>[2x]AKVFQWFGSNESGAEFGSQNLPGVEGKDYIWPDPNTIDTLISKGMNIFRVPFMMERLVPNSMTGSPDPNYLADLIATVNAITQKGAYAVVDPHNYGRYYNSIISSPSDFETFWKTVASQFASNPLVIFDTDNEYHDMDQTLVLNLNQAAIDGIRSAGATSQYIFVEGNSWTGAWTWTNVNDNMKSLTDPSDKIIYEMHQYLDSD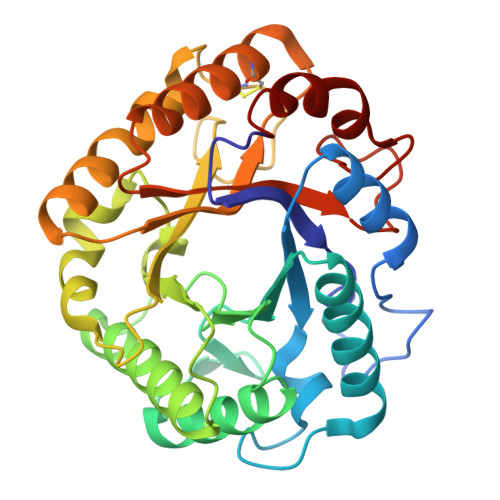GSGTSATCVSSTIGQERITSATQWLRANGKKGIIGEFAGGADNVCETAITGMLDYMAQNTDVWTGAIWWAAGPWWGDYIFSMEPDNGIAYQQILPILTPYL> RPESELIRQSWRVVSRSPLEHGTVLFARLFALEPSLLPLFQYNGRQFSSPEDSLSSPEFLDHIRKVMLVIDAAVTNVEDLSSLEEYLTSLGRKHRAVGVRLSSF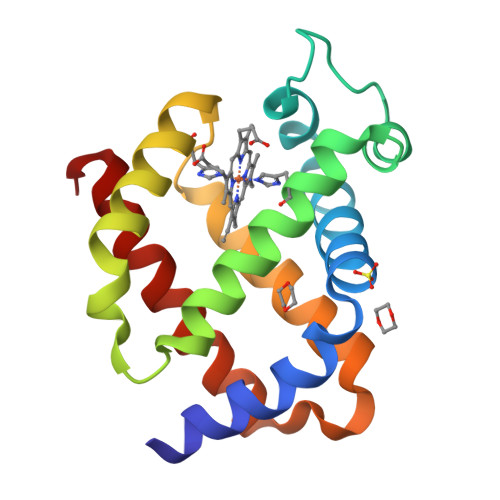STVGESLLYMLEKSLGPDFTPATRTAWSRLYGAVVQAMSRGWDG>[2x]SKVMTLKDAIAKYVHSGDHIALGGFTTDRKPYAAVFEILRQGITDLTGLGGAAGGDWDMLIGNGRVKAYINCYTANSGVTNVSRRFRKWFEAGKLTMEDYSQDVIYMMWHAAALGLPFLPVTLMQGSGLTDEWGISKEVRKTLDKVPDDKFKYIDNPFKPGEKVVAVPVPQVDVAIIHAQQASPDGTVRIWGGKFQDVDIAEAAKYTIVTCEEIISDEEIRRDPTKNDIPGMCVDAVVLAPYGAHPSQCYGLYDYDNPFLKVYDKVSKTQEDFDAFCKEWVFDLKDHDEYLNKLGATRLINLKVVPGLGYHIDMTKE;>[2x]DYTNYTNKEMQAVTIAKQIKNGQVVTVGTGLPLIGASVAKR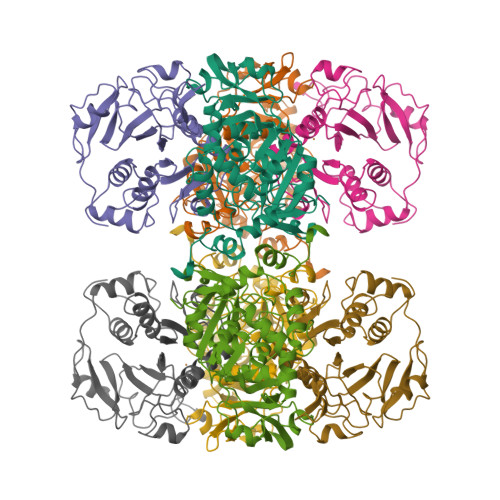VYAPDCHIIVESGLMDCSPVEVPRSVGDLRFMAHCGCIWPNVRFVGFEINEYLHKANRLIAFIGGAQIDPYGNVNSTSIGDYHHPKTRFTGSGGANGIATYSNTIIMMQHEKRRFMNKIDYVTSPGWIDGPGGRERLGLPGDVGPQLVVTDKGILKFDEKTKRMYLAAYYPTSSPEDVLENTGFDLDVSKAVELEAPDPAVIKLIREEIDPGQAFIQVP>[2x]HMNATVETTQHDVEGTGAAGATAMLFPGMGPAAFSDVGRFMVTNRYTRELLAEADDTLGYSLVDRFRQAEGDYSEYAQIAFLVNCVALARWAEQTMDLTPRICAGACFGEKSVAAYSGALTFADAVRMTAGLARCMD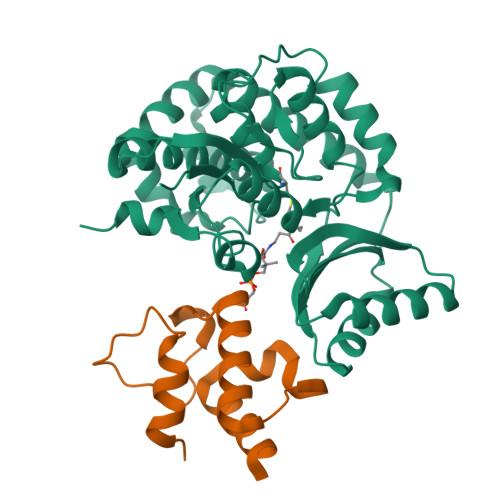EYFRTEHLGVVTHSFVRAPRERLDEILAELDERGEWHEISCHIDHDFFMLTLHERNSVWLEGRLRSVGAMPLYAMRPPMHAAAFGGLRDKAEEEVIAPLTFHDPTLPVVADQDGKVLTTGDEVRTMLLESFVRPLRWPDVISSLQDQGVTRVCVAGPDSLFGRVGTTTRAFEVIAATPRLALQPRARTTSR;>GSHMWDAQFENLLRRYLPFLSADQPLEQDINLRDIGLDSLGTVELLSELENTYDVHFQDEALTKETFETPGVLWKTLSQMVEPRH[2x]> APLTYELPDETAQLKPAPQPGFEAAQNNCAACHSVD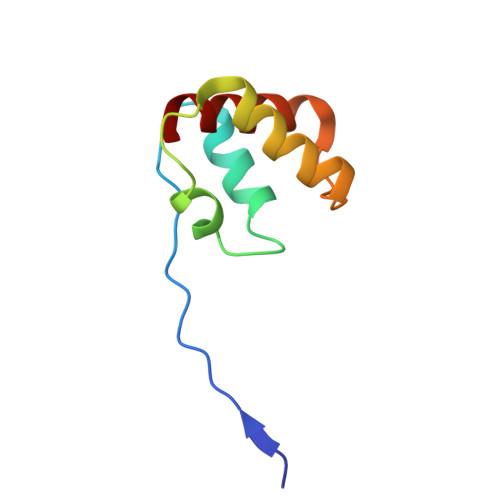YINTQPPGKGQAFWDAEVQKMIKVYHAPVDEADAKAIADYLAKTY> MSTISYIYWDDFSRFSYNFGTKLQFLGKSVCFENPLAPSSTNLYTWSSQTNYQSKRISPNLPLLRKGTRYSLSLNAELDLVSSLFVRIEFYNRFNESVGFELLKKDSIIFIYPKEAYTYTISLINAGCSDFTFHYLKLEEVTDSVIQEKNLSTEFTIEEHQDVLNLLLVEKKDSVYINKIESISQLQQKVELVSNPSLNSDSLILPELEKGLEDALKVFPNIKINVIAYGTQ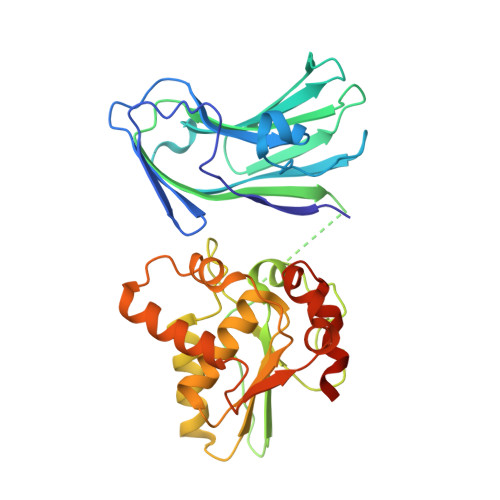GNFAALYYAKKFPRITAYINDCFAPFGILLKSLPHLTAKQQIFLREVWDTRETSPNVKHYGLVSENSSLNLVSMILSGNEHLPYLTLLKKQDDNYDSL> GSPDLAARTTMFEI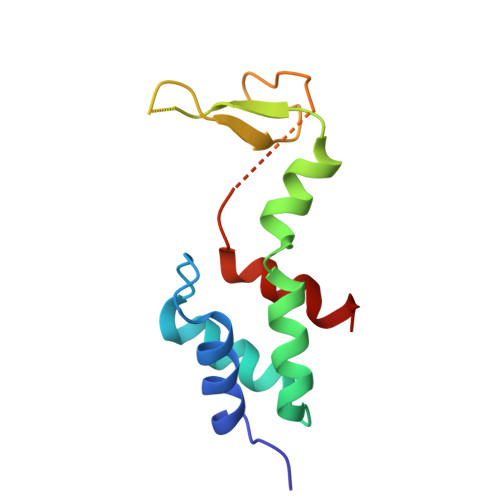NVGDTPCVLTKEDYRTLGAMTEGYSGSDIAVVVKDALMQPIRKIQSATHFKDVSTEDDETRKLTPCSPGDDGAIEMSWTDIEADELKEPDLTIKDFLKAIKST>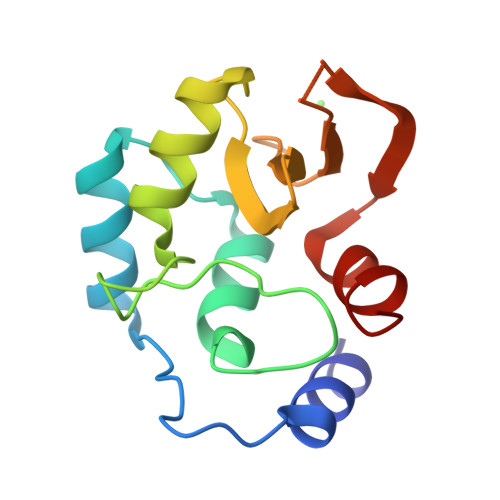 LEEVIEQLREANEPVPVPLELPDEDQLVEIEEQLFINIPFVFKEFLLTVSDVVYGSLEPVTVTDPQSHTYLPEVCATAWDLGVPRELIPICQDGEDYYCVEEDGTVLLWSAEEELVTEESWESVWHWARDVWLES>APDTSVSNKQNFSTDVIYQIFTDRFSDGNPANNPTGAAFDGSCTNLRLYCGGDWQGIINKINDGYLTGMGITAIWISQPVENIYSVINYSGVNNTAYHGYWARDFKKTNPAYGTMQDFKNLIDTAHAHNIKVIIDFAPNHTSPASSDDPSFAENGRLYDNGNLLGGYTNDTQNLFHHYGGTDFS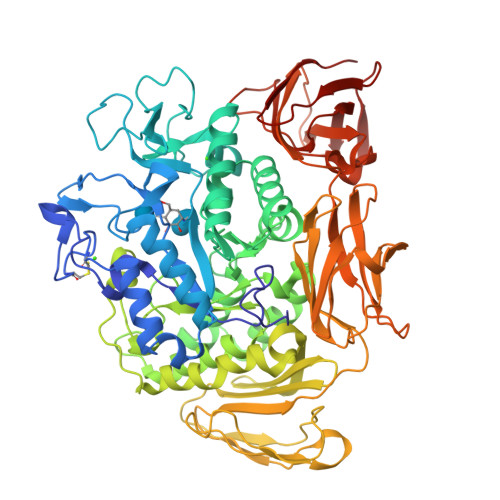TIENGIYKNLYDLADLNHNNSSVDVYLKDAIKMWLDLGVDGIRVDAVKHMPFGWQKSFMATINNYKPVFTFGEWFLGVNEISPEYHQFANESGMSLLDFRFAQKARQVFRDNTDNMYGLKAMLEGSEVDYAQVNDQVTFIDNHDMERFHTSNGDRRKLEQALAFTLTSRGVPAIYYGSEQYMSGGNDPDNRARLPSFSTTTTAYQVIQKLAPLRKSNPAIAYGSTHERWINNDVIIYERKFGNNVAVVAINRNMNTPASITGLVTSLPRGSYNDVLGGILNGNTLTVGAGGAASNFTLAPGGTAVWQYTTDATTPIIGNVGPMMAKPGVTITIDGRGFGSGKGTVYFGTTAVTGADIVAWEDTQIQVKIPAVPGGIYDIRVANAAGAASNIYDNFEVLTGDQVTVRFVINNATTALGQNVFLTGNVSELGNWDPNNAIGPMYNQVVYQYPTWYYDVSVPAGQTIEFKFLKKQGSTVTWEGGANRTFTTPTSGTATVNVNWQP[2x]> MKITVLGCGALGQLWLTALCKQGHEVQGWLRVPQPYCSVNLVETDGSIFNESLTANDPDFLATSDLLLVTLKAWQVSDAVKSLASTLPVTTPILLIHNGMGTIEELQNIQQPLLMGTTTHAARRDGNVIIHVANGITHIGPARQQDGDYSYLADILQTVLPDVAWHNNIRAELWRKLAVNCVINPLTAIWNCPNGELRHHPQEIMQICEEVAAVIEREGHHTSAEDLRDYVMQVIDATAENISSMLQDIRALRHTEIDYINGFLLRRARAHGIAVPENTRLFEMVKRKESEYERIGT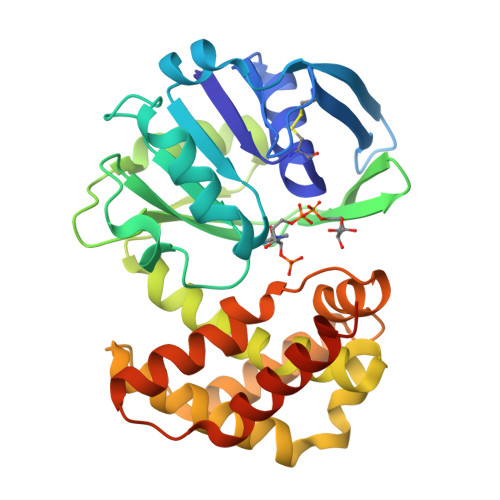GLPRPW> SVATV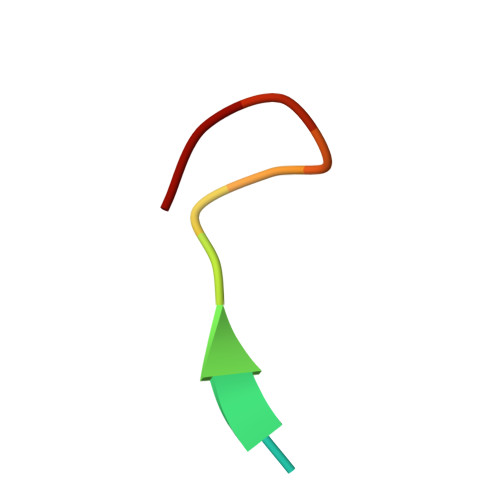SESLLTE>[2x]QVAEDCMGLLQLLSNGTVLRSESIDLITQQIPFKNNQTVLFKDSIYHKPNNLHLRLYKPISASNRTALPVVVFFHGGGFCFGSRSWPHFHNFCL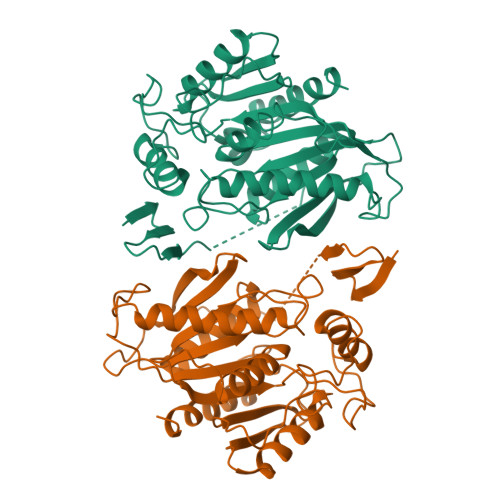TLASSLNALVVSPDYRLAPEHRLPAAFEDAEAVLTWLWDQAVSDGVNHWFEDGTDVDFDRVFVVGDSSGGNIAHQLAVRFGSGSIELTPVRVRGYVLMGPFFGGEERTNSENGPSEALLSLDLLDKFWRLSLPNGATRDHHMANPFGPTSPTLESISLEPMLVIVGGSELLRDRAKEYAYKLKKMGGKRVDYIEFENKEHGFYSNYPSSEAAEQVLRIIGDFMNNLS>[2x]SNAMANIKIRQETPTAFYIKVHDTDNVAIIVNDNGLKAGTRFPDGLELIEHIPQG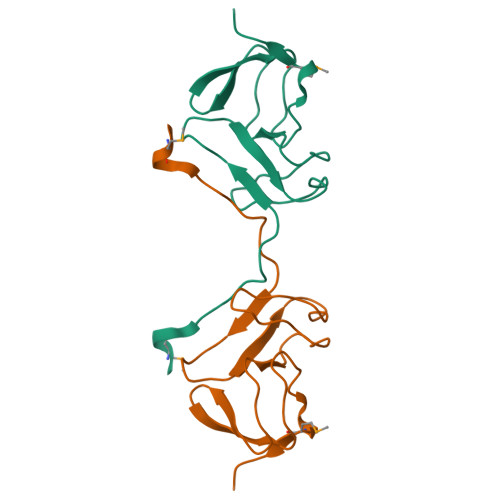HKVALLDIPANGEIIRYGEVIGYAVRAIPRGSWIDESMVVLPEA>DLKLDDLKSLTAGSGQQEIEQTINKYSNMLTSIVSSLQEDERGGSAITVHDVGGKKSQYLEKINEVIRRAWAVPTHGHELGYSLCNSLRQSGGLDLLMKNCVKPDLQFSSAQLLEQCLTTENRKHVVDNGLDKVVNVACVCTKNSNMEHSRVGTGILEHLFKHSEGTCSDVIRLGGLDAVLFECRTSDLETLRHCASALANLSLYGGAENQEEMILRKVPMWLFPLAFHNDDNIKYYACLAIAVLVANKEIEAEVLKSGCLDLVEPFVT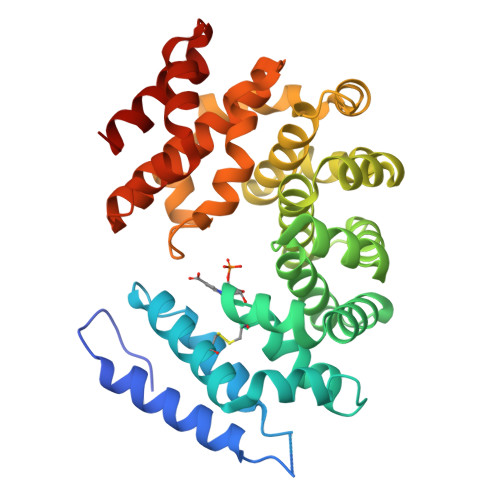SHDPSAFARSNLAHAHGQSKHWLKRLVPVLSSNREEARNLAAFHFCMEAGIKREQGNTDIFREINAIEALKNVASCPNAIASKFAAQALRLIGET[3x]>[2x]MFHSSAMVNSHRKPMFNIHRGFYCLTAILPQICICSQFSVPSSYHFTEDPGAFPVATNGERFPWQELRLPSVVIPLHYDLFVHPNLTSLDFVASEKIEVLVSNATQFIILHSKDLEITNATLQSEEDSRYMKPGKELKVLSYPAHEQIALLVPEKLTPHLKYYVAMDFQAKLGDGFEGFYKSTYRTLGGETRILAVTDFEPTQARMAFPCFDEPLFKANFSIKIRRESRHIALSNMPK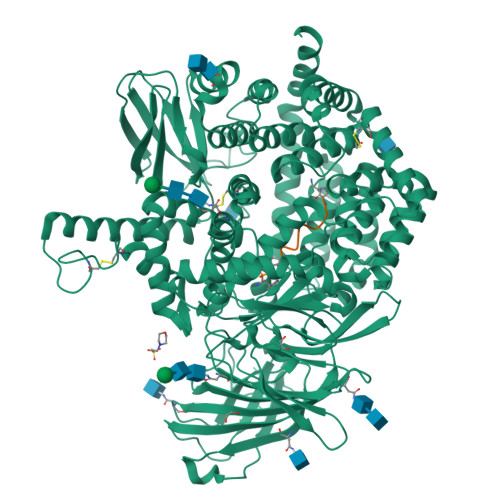VKTIELEGGLLEDHFETTVKMSTYLVAYIVCDFHSLSGFTSSGVKVSIYASPDKRNQTHYALQASLKLLDFYEKYFDIYYPLSKLDLIAIPDFAPGAMENWGLITYRETSLLFDPKTSSASDKLWVTRVIAHELAHQWFGNLVTMEWWNDIWLNEGFAKYMELIAVNATYPELQFDDYFLNVCFEVITKDSLNSSRPISKPAETPTQIQEMFDEVSYNKGACILNMLKDFLGEEKFQKGIIQYLKKFSYRNAKNDDLWSSLSNSCLESDFTSGGVCHSDPKMTSNMLAFLGENAEVKEMMTTWTLQKGIPLLVVKQDGCSLRLQQERFLQGVFQEDPEWRALQERYLWHIPLTYSTSSSNVIHRHILKSKTDTLDLPEKTSWVKFNVDSNGYYIVHYEGHGWDQLITQLNQNHTLLRPKDRVGLIHDVFQLVGAGRLTLDKALDMTYYLQHETSSPALLEGLSYLESFYHMMDRRNISDISENLKRYLLQYFKPVIDRQSWSDKGSVWDRMLRSALLKLACDLNHAPCIQKAAELFSQWMESSGKLNIPTDVLKIVYSVGAQTTAGWNYLLEQYELSMSSAEQNKILYALSTSKHQEKLLKLIELGMEGKVIKTQNLAALLHAIARRPKGQQLAWDFVRENWTHLLKKFDLGSYDIRMIISGTTAHFSSKDKLQEVKLFFESLEAQGSHLDIFQTVLETITKNIKWLEKNLPTLRTWLMVNTRHHHHHH;>XXKHHAFSFK[2x]>GSSHHHHHHENLYFQSMFGPEHAEVYEAAYRGRGKSWHDEAADVADRIRAARPDAARLLDVGCG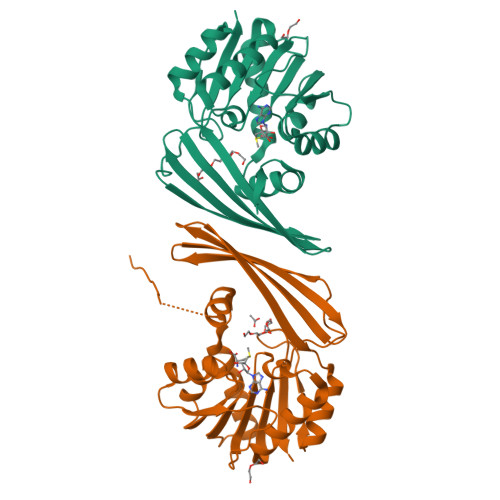TGAHLETFATRFPHVEGLELAPAMLALARHRLPGVRLHAGDMRTFDLGVTFDAVTCLFTAVNFLGTVAEMRAAVAAMSAHLAPGGVLVLEPWWFPERFIDGYVGGDLVREEGRTVARVSRSTRQGRVTRMEERWLVGDAAGIREFSQVGLLTMFTREEYDAAFAAAGCESAYVEGWLTGRGLFVATRTGGHATPTMV[2x]The transfer of an acetyl group from acetyl-coenzyme A to the free α-amino group on the N-terminus of substrate proteins is catalyzed by N-terminal acetyltransferases (NATs), and is considered to be irreversible, as no Nt-deacetylase has been identified so far. NatC acetylates protein N-termini starting with methionine, followed by a hydrophobic or amphipathic amino acid, with amino acids at positions 3 and 4 also contributing to NatC recognition. NatC forms a heterotrimeric complex, containing the catalytic subunit Naa30, the small auxiliary subunit Naa38 and the large auxiliary subunit Naa35. The large auxiliary subunit Naa35 acts as the central assembly hub of the NatC complex, forming extensive interactions with Naa30 and Naa38.

To obtain insights into the substrate recognition mode and the marked difference of NatC catalytic efficiencies toward the two peptides, crystal structures of NatC in complex with CoA, and either yArl3 or Gag peptide were determined to a maximal resolution of 2.99 and 2.75 Å, respectively. The electron density of the peptide ligands was sufficient to model the first four and six amino acids of the yArl3 and Gag peptide, respectively. The yArl3 and the Gag peptide formed several side chain and backbone interactions, mostly with Naa30, but also with Naa35. In both structures, the methionine sulfur atom at peptide position 1 is within hydrogen bond distance to Ser28. The Phe2 and Leu2 side chains of the yArl3 and Gag peptide, respectively, were positioned in a hydrophobic pocket (the “main peptide pocket”), which is formed by conserved residues from α2 and β4 of Naa30, as well as the short 310-helix η3 from Naa35. In the yArl3-bound structure, in contrast, Naa30-Glu29 forms an alternative hydrogen bond with yArl3-His3 and does not contact the peptide backbone. The yArl3-Leu4 side chain is at the periphery of this pocket. The α1–α2 loop of Naa30 moved ~2.8 or 3.5 Å upon binding of the yArl3 or Gag peptide, respectively. In contrast, the Leu27 side chain appears to be flexible in the yArl3 structure. For the yArl3 peptide, this interaction is sterically prevented by a hydrogen bond of yArl3-His3 with Naa30-Glu29, which may partially account for the reduced specificity constant of yArl3 compared to Gag.

> MEIVYKPLDIRNEEQFASIKKLIDADLSEPYSIYVYRYFLNQWPELTYIAVDNKSGTPNIPIGCIVCKMDPHRNVRLRGYIGMLAVESTYRGHGIAKKLVEIAIDKMQREHCDEIMLETEVENSAALNLYEGMGFIRMKRMFRYYLNEGDAFKLILPLT;> GPMEVDSILGSLSITDDFDQLVDVTSLFDELCSKLKPEAIVKDPRFDLFEGTHSLEVNNSKLDSSLIELTAEEIEFDVNVAYDPPLASVAAIADRLLRCVISWLNDYQTLPTTVLSCRYTESLLSSLVKGTTAGSSWCTGNILYDKVLGSCILGVCYLTKFVQKLLSAGIVFEEEDLNFNNMGFNTFDNLPGQDVVINSLTESLQILEAYSDDSLHLTMLKHILKIIICLVHLEDHLTDYSTKTSHLDELIENANSVNGIFPQLQLSPPKGAFSTYIQKHRSNQFPPRKITKLPTDYSGFITLANDVKTILLVDKAESALETYQFAKFFNKLEQRHVIARILFPLFFIRDDRTVLGKFSYTQFYLLHVKEFSAQTPSEFESSIGNELIQESSNMLLEWYQNCSQNTCRYRQGFNRQLILWDSLQAQFESVNSQVYCSWTYFMKLSSMIEFSLKGFDLDIYKPFEAYSMFWYVYYLSHHLETFLKDSQNDIESNINAIHSMNKKLKKLKAGEKKDQLRLKYRFAMDNEMEQLQATKQFLNYLLKEINITKSLCLIEVFQFAILKSFGLIDNKNSTPSKFSNERLIHNLRFKPFNSIGVPELPEYEVFQQTLKDFVIEEKGAAFDIKLERATNFIETEVRNVVSSIDEIMQGIKGGDNNGVLVTGTRLVQELSLEYYCKLKHTSKALSVNSKVIVNTLKKNIKNKDSHEYKVELVHTTEGWNYFPIQTLRIKQDRYK;> MDILKLSDFIGNTLIVSLTEDRILVGSLVAVDAQMNLLLDHVEERMGSSSRMMGLVSVPRRSVKTIMIDKPVLQELT;> MFHLVGSRRR ANTAR domains are a class of antiterminator that bind and stabilize dual hexaloop RNA motifs within the nascent RNA chain to prevent terminator loop formation. EutV possesses one of the most common domains architectures found among all ANTAR proteins annotated in the Pfam database, consisting of an N-terminal phosphor-sensitive REC domain (aa 1–119) coupled to a C-terminal ANTAR domain (aa 141–186) via a coiled-coil domain. Ethanolamine (EA) stimulates the histidine kinase EutW (component 1) to phosphorylate EutV (component 2) which promotes homodimerization of the protein. Dimeric EutV acts as an antiterminator of RNAP by binding these dual hexaloop motifs within the nascent mRNA chain inhibiting T-loop formation and thereby preventing transcription termination.

Within the crystal, EutV showed a symmetric dimer ‘dumbbell’ conformation with 48 residues contributing to 1870 A2 of buried surface area and extensive hydrophobic and ionic interactions between residues Ser85 and Glu161 of each chain. The REC domain of each chain dimerized through a common ‘α4-β5-α5’ mode forming one end of the dumbbell with the ANTAR domains forming the other end. The handle of the dumbbell consists of a coiled-coil that includes residues Leu128, Ile132, Leu135 and Leu139 and forms the majority of hydrophobic interactions within a heptad repeat. The interaction between the two ANTAR domains is stabilized by mutual hydrogen bonds between Arg142 to Glu146 (2.9 and 3.0 Å), and the amine group of chain a Glu161 to Glu160 chain b (3.1 Å). The dimeric state within the crystal structure was unexpected given the recombinant EutV used for crystallography was not phosphorylated nor supplemented with phosphomimetics. SEC-MALS analysis performed in this work indicated EutV was largely monomeric in solution although may form higher order species, likely a dimer at increased concentrations. In this way, during crystallization and with an increased concentration of EutV, the dimeric state was likely preferentially favoured. The dimeric RNA-free structure of EutV resembles the crystal structure of the ANTAR domain protein AmiR from P. aeruginosa. Within the EutV structure, the conserved active site residues in the N-terminal REC domain are in a ‘phospho-activated’ state, as indicated by their position relative to the to the BeF3– activated CheY/CheZ complex and the BeF3– activated EutV bound RNA structure. This positioning indicates that the dimeric structure of EutV observed in the crystal is representative of the biologically active phosphorylated dimer required for efficient antitermination.

>[2x]SNMDGRIVIVDDEPITRLDIRDIVIEAGYEVVGEAADGFEAIEVCKKTQPDLVLMDIQMPILDGLKAGKKIVQDQLASSIVFLSAYSDVQNTDKAKKLGALGYLVKPLDEKSLIPTIEMSIERGKQTQLLLSQIDKLSLKLEERKIIEKAKGILVKENHISEEEAYQMLRTLSMNKRARMSEIAELIVMDDE>MVPGACPLILRLSPTLHSADLIRDIDAMRWFLFEDTGVPLPEVNIEVLPEPTEKLTVLLYQEPVFSLSIPAQADYLLIGADASVVGDSQTLPNGMGQICWLTKDMAHKAQGFGLDVFAGSQRISALLKCVLLRHMGEFIGVQETRYLMNAMEKNYSELVKELQRQLPINKIAETLQRLVSERVSIRDLRLIFGTLIDWAPREKDVLMLTEYVRIALRRHILRRLNPEGKPLPILRIGEGIENLVRESIRQTAMGTYTALSSRHKTQILQLIEQALKQSAKLFIVTSVDTRRFLRKITEATLFD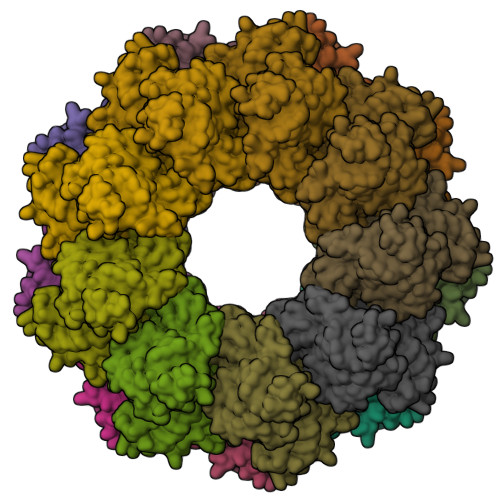VPILSWQELGEESLIQVVESIDLSEEELADNEE[18x]The TNA backbone is composed of phosphodiester-linked 3′→2′ α-l-threofuranose sugars and, therefore, has one fewer atom in its repeating unit than RNA. Critically, TNA can form stable Watson−Crick duplexes with itself, DNA and RNA, such that the exchange of genetic information between these polymers appears feasible. Here, we examine the behaviour of TNA in nonenzymatic template-directed primer extension reactions from both a kinetic and a structural perspective. Taken together, we propose that structural constraints explain the diminished ability of TNA to engage in nonenzymatic template-directed primer extension, and we discuss the consequences of these observations for the plausibility of the involvement of TNA in the origin of primitive cells.

We first co-crystallized the unactivated α-l-threofuranosylguanine-3′-monophosphate (tGMP) monomer with a short partially self-complementary RNA 7-mer (TNA-M1, sequence: 5′-mCmUGUACA-3′, italic: locked nucleotides, mC: locked 5-methylcytidine, mU: locked 5-methyluridine). This oligonucleotide self-anneals to form a central six base pair duplex, flanked by single overhanging 5-Me-C residues, to which the complementary G or tG monomer can bind. When incubated with tGMP, crystals grew in the hexagonal P63 space group, and we determined the structure to a resolution of 2.36 Å. Similar to our previously reported RNA-GMP complex structure, the helical duplexes are end-to-end stacked, and a tGMP nucleotide is bound to the templating 5-methylcytidine residue at each end in a Watson-Crick base pair. The sugar is in the C4′-exo conformation in both tGMP ligands. The well-defined electron density of the 3′-phosphate of tGMP shows that the distance between the 3′-OH of the RNA primer and the phosphorus atom of tGMP is ∼6.7 Å, slightly longer than the distance observed for the ribo-nucleotide monomer (∼6.3 Å). In both structures, the longer distance between the primer 3′-OH and the bound tGMP monomer appears to be influenced by the structure of the threo-nucleotide, in which the phosphate group is directly attached to the threo-furanosyl ring instead of being held away from the sugar by the 5′-methylene of ribose. One noteworthy conformational difference between complexes TNA-M1 and TNA-M2 is that the bound monomers have χ torsion angles that differ by >40°. Without any helper to enhance the binding, the χ angle of tGMP in TNA-M1 is –177°, which is closer to the characteristic χ torsion angle in an A-form helix. In the absence of covalent linkage to the RNA backbone at either the 3′ or 2′ terminus, the tGMP monomers in both TNA-M1 and TNA-M2 complexes may be in a more relaxed conformation, to differing extents depending on the presence of a proximal downstream oligonucleotide.

>NUGUACA[2x]>[5x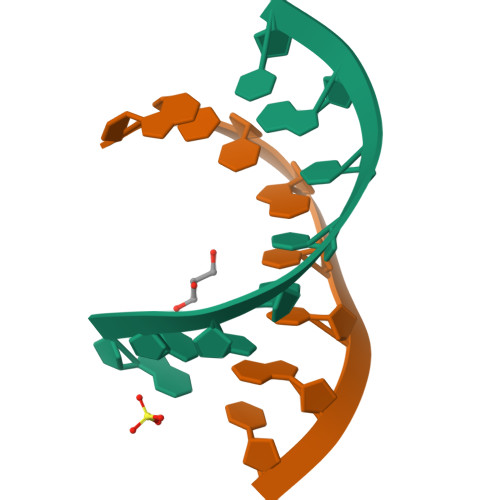]GCUGCUGC> GDVQNAVEGAMVRVADTVQTSATNSERVPNLTAVETGHTSQAVPGDTMQTRHVINNHVRSESTIENFLARSACVFYLEYKTGTKEDSNSFNNWVITTRRVAQLRRKLEMFTYLRFDMEITVVITSSQDQSTSQNQNAPVLTHQIMYVPPGGPIPVSVDDYSWQTSTNPSIFWTEGNAPARMSIPFISIGNAYSNFYDGWSHFSQAGVYG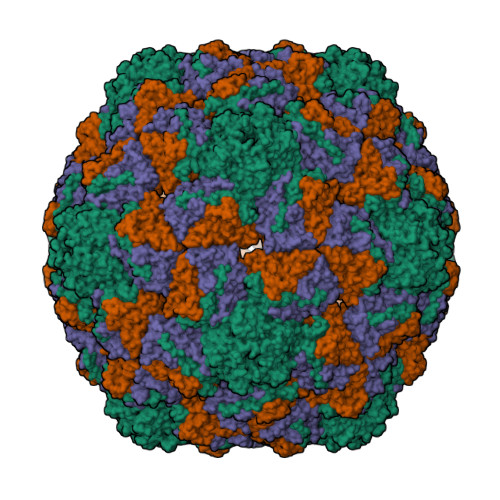FTTLNNMGQLFFRHVNKPNPAAITSVARIYFKPKHVRAWVPRPPRLCPYINSTNVNFEPKPVTEVRTNIITT;> GYSDRVRSITLGNSTITTQECANVVVGYGEWPEYLSDNEATAEDQPTQPDVATCRFYTLDSVQWENGSPGWWWKFPDALRDMGLFGQNMYYHYLGRAGYTIHVQCNASKFHQGCILVVCVPEAEMGSAQTSGVVNYEHISKGEIASRFTTTTTAEDHGVQAAVWNAGMGVGVGNLTIFPHQWINLRTNNSATIVMPYVNSVPMDNMYRHHNFTLMIIPFVPLDFSAGASTYVPITVTVAPMCAEYNGLRLAGHQ;> GLPTMNTPGSNQFLTSDDFQSPSAMPQFDVTPEMHIPGEVRNLMEIAEVDSVMPINNDSAAKVSSMEAYRVELSTNTNAGTQVFGFQLNPGAESVMNRTLMGEILNYYAHWSGSIKITFVFCGSAMTTGKFLLSYAPPGAGAPKTRKDAMLGTHVVWDVGLQSSCVLCIPWISQTHYRFVEKDPYTNAGFVTCWYQTSVVSPASNQPKCYMMCMVSACNDFSVRMLRDTKFIEQTSFYQ>[4x]MFLAPWIERRLRYHPTIELPDDTRGHILIFGIDPITRTLIRKLESRNHLFVVVTDNYDQALHLEEQEGFKVVYGSPTDAHVLAGLRVAAARSIIANLSDPDNANLCLTVRSLCQTPIIAVVKEPVHGELLRLAGANQVVPLTRILGRYLGIRATTCGALAHILDSFGNLQIAELPVHGTPFAGKTIGESGIRQRTGLSIIGVWERGSLTTPQRETVLTEQSLLVLAGTKSQLAALEYLIGEAPEDELIFIIGHGRIGCAAAAFLDRKPVPFILIDRQESPVCNDHVVVYGDATVGQTLRQAGIDRASGIIVTTNDDSTNIFLTLACRHLHSHIRIVARANGEENVDQLYAAGADFVVSNASVGANILGNLLEHKESAFLSEGMAVFRRPLPPAMAGKTIAETRLRPLTGCSIVAIEAPDRADILISPPPETILAEGARLILIGTSEQEKTFDQTIAARLVPR

Each GsuK subunit contains two tandem RCK domains, reminiscent of Slo K+ channels. We demonstrate that GsuK is a nucleotide-activated and Ca2+-deactivated K+ channel and reveal the structural mechanism of multi-ligand gating of this double-RCK K+ channel and a distinct pore opening mechanics. Ca2+ stabilizes the closed gating ring by binding at the inter-subunit assembly interfaces and deactivates the GsuK channel. While both NAD+ and ADP anchor their adenine rings at the same site on RCK2 by using the conserved nucleotide binding motif, they utilize different functional groups and activate the channel at different sites.

Our study of GsuK started with the structure determination of its two tandem RCK domains, labeled as RCK1 and RCK2. The two intracellular ligand binding RCK domains form a bi-lobed structure equivalent to the MthK RCK dimer; each lobe consists of the N-terminal two-thirds of the RCK domain (βA to αF) and adopts a Rossmann-fold. In GsuK, the equivalent αG helix is absent in RCK1 and becomes a shorter helix with a different orientation in RCK2, resulting in swapped and loosely packed C-terminal subdomains. The pore-connecting top half of the GsuK gating ring is in a contracted form similar to the closed MthK whereas the bottom half is more expanded, suggesting that the structure likely represents a closed conformation. Furthermore, each subunit also contains a small fragment of the pore-lining inner helix at its N-terminus, which forms a short four-helix bundle atop the center of the gating ring and creates a constriction point at the intracellular end of the pore that would occlude the passage of hydrated K+ ions. The helix bundle is tethered to RCK1 by linkers in an extended configuration, ensuring a tight coupling between the gating ring conformational change and pore opening at the intracellular gate. Indeed, electron density modeled as AMP was observed at the predicted nucleotide binding site in the GsuK gating ring structure. As no nucleotides were added during protein purification or crystallization, the bound nucleotide is likely from the E. coli cells used for protein expression. Two bound metal ions were observed in each GsuK subunit. The second bound ion, identified as Ca2+ based on ligand chemistry and functional assays, is positioned at the inter-subunit assembly interface, a location reminiscent of the Ca2+ bowl in BK channel.>KPKLLNKFDKTIKAELDAAEKLRKRGKIEEAVNAFKELVRKYPQSPRARYGKAQCEDDLAEKRRSNEVLRGAIETYQEVASLPDVPADLLKLSLKRRSDRQQFLGHMRGSLLTLQRLVQLFPNDTSLKNDLGVGYLLIGDNDNAKKVYEEVLSVTPNDGFAKVHYGFILKAQNKIAESIPYLKEGIESGDPGTDDGRFYFHLGDAMQRVGNKEAYKWYELGHKRGHFASVWQRSLYNVNGLKAQPWWTPKETGYTELVKSLERNWKLIRDEGLAVMDKAKGLFLPEDENLREKGDWSQFTLWQQGRRNENACKGAPKTCTLLEKFPETTGCRRGQIKYSIMHPGTHVWPHTGPTNCRLRMHLGLVIPKEGCKIRCANETKTWEEGKVLIFDDSFEHEVWQDASSFRLIFIVDVWHPELTPQQRRSLPAI[2x];> AKDGLGEYTCTSLEGFEGK

Here, we report crystallographic and biochemical results on the structure and substrate selectivity of AspH. The results reveal a key role for the TPR domain of AspH in substrate binding and, unexpectedly, that the preferred EGFD-substrates of AspH have a non-canonical (Cys3–4) disulfide pattern. Whilst the oxygenase domain fold of AspH is typical for the 2OG oxygenase superfamily, details of its active site and the role of the TPR domain in EGFD-substrate binding are remarkable. Whatever the precise extent of conformational changes during catalysis, the results reveal a central role for the TPR domain in enabling AspH catalysis—without it, 2OG turnover occurs, but EGFDs are not hydroxylated.

We thus synthesised an irreversibly-linked cyclic analogue of the Cys3–4 EGFD disulfide substrate; A 10mer cyclic peptide (CP101–110) comprising the core residues (aa 101–110) of hFX EGF139mer, wherein the Cys3–4 disulfide was replaced by a stable thioether, was prepared using the method of Suga et al.. CP101–110 was efficiently Asp-β-hydroxylated by AspH-TPR-Ox (~85%), whereas cyclic peptides with variations in consensus sequence residues or a linear 10mer peptide were not, further supporting the crystallographically observed Cys3–4 disulfide as the preferred substrate form for AspH catalysis. An extended 19mer CP (CP101–119) was designed based on the enzyme-substrate contacts observed in the AspH-TPR-Ox:hFX structure and found to be a better substrate than CP101–110 (>95%). A structure of AspH co-crystallised with the CP101–119 (AspH-TPR-Ox:CP101–119) reveals this substrate bound to one of the two AspH molecules in the asymmetric unit (chain A). Conformational differences between the bound (chain A) and unbound (chain B) (Cα RMSD 3.82 Å) are consistent with afore-described observations implying an AspH induced fit mechanism with hFX.>[4x]SLTVKAYLLGKEDAAREIRRFSFCCSPEPEAEAEAAAGPGPCERLLSRV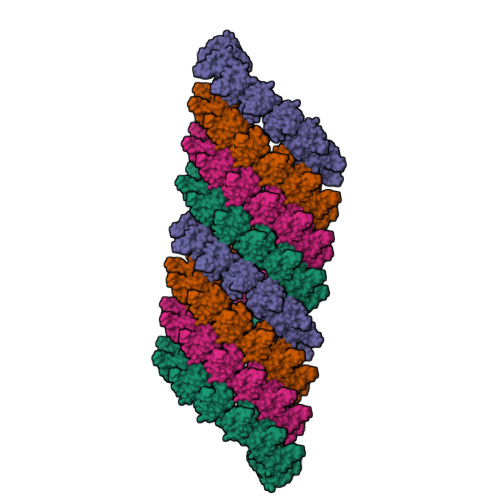AALFPALRPGGFQAHYRDEDGDLVAFSSDEELTMAMSYVKDDIFRIYIKEK> MMKIGVFVPIGNNGW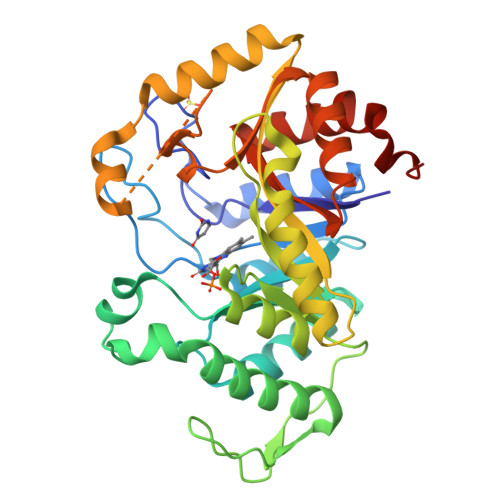LISTHAPQYMPTFELNKAIVQKAEHYHFDFALSMIKLRGFGGKTEFWDHNLESFTLMAGLAAVTSRIQIYATAATLTLPPAIVARMAATIDSISGGRFGVNLVTGWQKPEYEQMGIWPGDDYFSRRYDYLTEYVQVLRDLWGTGKSDFKGDFFTMNDCRVSPQPSVPMKVICAGQSDAGMAFSARYADFNFCFGKGVNTPTAFAPTAARMKQAAEQTGRDVGSYVLFMVIADETDDAARAKWEHYKAGADEEALSWLTEQSQKDTRSGTDTNVRQMADPTSAVNINMGTLVGSYASVARMLDEVASVPGAEGVLLTFDDFLSGIETFGERIQPLMQCRAHLPALTQEVA>[2x]MEKRMSTQQRAAGNACPTAAFSFDPARLAQRRRWAGAFAALCGLALSPSALLAEEHSQHQDHAVELAPSVVTGVAQSSPLTIVTNPKEPRQPVPASDGADYLKTIPGFAVIRNGGSNGDPVLRGMFGSRLNILTNGGMMLGACPNRMDAPTSYISPETYDKLTVIKGPQTVLWGPGASAGTILFEREPERFGELGSRVNASLLAGSNGRFDKVLDAAAGNRLGYLRFTGNHAQSDDYEDGAGNTVPSRWKKWNGDVAVGWTPDEDTLIELTAGKGDGEARYAGRGMDGSQFKRESLGLRFVKSNVSDVLEKVEAQVYYNYADAIMDNFRLRTPDPSSMMPMPMASQVDRRTLGGRLAATWRWDDFKLVTGVDAMRNEHRARGSKYDMMTDYYTDADQFPWSKDAVFHNYGAFGELTWFAAERDRLIGGLRLDRASVKDYRQTLKSGHMGHAMANPTANDTRADTLPSGFVRYEHDLADSPTTLYAGLGHAERFPDYWELFSPKRGPNGSVNAFDKIKPEKTTQLDFGLQYNGDKLQAWASGYVGVVQDFILFSYREGMMGSSTQATNVDARIMGGELGASYQLTGNWKTDASLAYAWGKNSSDDRALPQIPPLEARFGLTYEEGDWSAGSLWRVVAPQNRIARDQGNVVGKDFDKSAGFGVFSLNGAYRVTRNVKLSAGVDNLFDKDYTEHLNKAGDAGFGFSANETVPEPGRTFWTKVDFSF

Here, we show that Pseudomonas aeruginosa OprC is an outer membrane, TonB-dependent transporter that is conserved in many Proteobacteria and which mediates acquisition of both reduced and oxidised ionic copper via an unprecedented CxxxM-HxM metal binding site. As indicated by the successful structure solution, OprC contains a single bound copper and shows the typical fold of a TBDT, with a large 22-stranded β-barrel occluded by an N-terminal approximately 15 kDa plug domain that, like in other TBDTs, completely occludes the lumen of the barrel. The copper binding site comprises residues Cys143 and Met147 in the plug domain and His323 and Met325 in the barrel wall. The CxxxM-HxM configuration, which coordinates the copper in a tetrahedral manner, is highly unusual and has, to our knowledge, not been observed before in copper homeostasis proteins.

While OprCWT and most single alanine mutants can be (partly) loaded via Cu(II) incubation, this is not the case for the C143A mutant. We hypothesised that removal of the cysteine could lead to much lower affinity for Cu(II), so that after SEC, nothing remains bound. To provide support for this, we determined the crystal structures of the OprC C143A mutant cocrystallised with Cu(II) or silver Ag(I). For each crystal, datasets were collected at 8,800 eV and 9,175 eV to distinguish between both metals. Bound copper is expected to give a strong anomalous peak only at 9,175 eV (which is above the copper K edge at 8,979 eV), while bound silver will give comparable peaks at both energies (the silver L-III edge is at 3,351 eV). For C143A cocrystallised with Cu(II), no anomalous peaks are visible at both energies, showing that Cu(II) binding is indeed abolished. Crucially, in the presence of silver, the same 3 anomalous peaks are visible as for WT OprC (compare Fig 3A and 3D), strongly suggesting that the C143A mutant can still bind Cu(I). All 4 residues in the OprC binding site contribute to copper binding, but not to the same extent and, in some cases, not equally for both copper redox states. This is illustrated by Cys143, which is essential for high-affinity Cu(II) binding but dispensable for Cu(I).> MTTTQTAKASRRARIERRTRESDIVIELDLDGTGQVAVDTGVPFYDHMLTALGSHASFDLTVRATGDVEIEAHH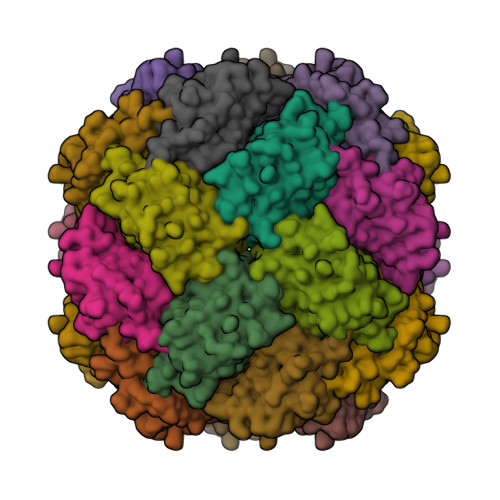TIEDTAIALGTALGQALGDKRGIRRFGDAFIPMDETLAHAAVDLSGRPYCVHTGEPDHLQHTTIAGSSVPYHTVINRHVFESLAANARIALHVRVLYGRDPHHITEAQYKAVARALRQAVEPDPRVSGVPSTKGAL>[2x]HMMAPEMDQFYRSTMAIYKSIMEQFNPALENLVYLGNNYLRAF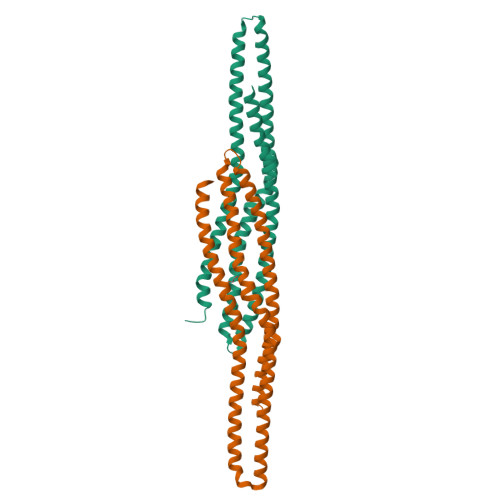HALSEAAEVYFSAIQKIGEQALQSSTSQILGEILVQMSDTQRHLNSDLEVVVQTFHGDLLQHMEKNTKLDMQFIKDSCQHYEIEYRHRAANLEKCMSELWRMERKRDKNAREMKESVNRLHAQMQAFVSESKRAAELEEKRRYRFLAEKHLLLSNTFLQFLGRARGMLQNRVLLWKEQS Hydroxysteroid 17-beta-dehydrogenase 13 (HSD17B13) is a hepatic lipid droplet-associated enzyme that is upregulated in patients with non-alcoholic fatty liver disease. Recently, there have been several reports that predicted loss of function variants in HSD17B13 protect against the progression of steatosis to non-alcoholic steatohepatitis with fibrosis and hepatocellular carcinoma. Here we report crystal structures of full length HSD17B13 in complex with its NAD+ cofactor, and with lipid/detergent molecules and small molecule inhibitors from two distinct series in the ligand binding pocket. The overall structure of each HSD17B13 subunit could be divided into two parts: (i) the catalytic core domain (residues 29–259) that contained the cofactor binding site and the catalytic center and (ii) the membrane anchoring domain that consisted of the N-terminal helix (N2-P28) which was highly hydrophobic and a C-terminal proximal helix-turn-helix motif (P260-N286) which formed an amphipathic patch on the protein surface.

Based on findings from dog HSD17B13 crystals, we changed four surface residues distant from the active site of human HSD17B13 to those of dog protein at the dog HSD17B13 crystal interface (Q60K, I62R, R71H, and E161K, human mutant) to improve the resolution of the human HSD17B13 crystals and obtained useful crystals of the human mutant HSD17B13 in complex with NAD+ and compound 2 (compound 2-human). The crystal of the compound 2-human HSD17B13 contained four HSD17B13 dimer complexes in the asymmetric unit, with 2 occupying all the protein subunits. In some subunits, long rod-shaped electron densities were observed together with those of 2 at the binding sites. We built detergent C12E8 molecules into these densities, but these densities could be from the alkyl chain of the solubilized endogenous phospholipids as well. Like 1, 2 binding also displaced the C-terminal peptides in HSD17B13. In detergent co-existing binding sites, these peptides, as extensions of the P274-N286 helices, shifted positions relative to those of the apo dog HSD17B13 to interact with bound C12E8 molecules. Like 1, the negatively charged carboxylate of 2 formed hydrogen bonds with S172 and Y185 and contacted the positively charged nicotinamide ring of NAD+ at closest distances of 3.1 Å to the C4N and C5N atoms. The terminal tosyl group extended toward the lipid membrane, interacting with the helix-turn-helix motif. While the terminal fluorophenyl of 1 pointed toward an opening that faces solvent, this opening was sealed by the extended P274-A291 helix in the 2 complex with detergent. Observations of lipid/detergent molecules in human HSD17B13/2 complex interacting with the N-terminal helices and the helix-turn-helix motifs directly demonstrated that these structural elements are indeed responsible for membrane anchoring.

>[8x]MGNIILEILLLLITIIYSYLESLVKFFIPQRRKSVAGEIVLITGAGHGIGRQTTYEFAKRKSRLVLWDINKHGVEETAAECRKLGVTAHAYVVDCSNREEIYRSLNQVKKEVGDVTIVVNNAGTVYPADLLSTKDEEITKTFEVNILGHFWITKALLPSMMKRNHGHIVTVASVCGHEGIPYLIPYCSSKFAAVGFHRGLTSELQALGKTGIKTSCLCPVFVNTGFTKNPSTRLWPVLETDEVVRSLIDGILTNKKMIFVPSYINIFLRLQKFLPERASAILNRMQNIQFEAVVGHKIKMKGSGHHHHHHHHHHH> MSGSHHHHHHSSGIEGRGRLQTRQDVLYLYNWTYYTPTSLIKKFEQQYNVQVVYDDYASNEDMFAKLSIGASGYDLVVPSGDFVSIMKRKHLLEKIDLSKIPNVQFIKES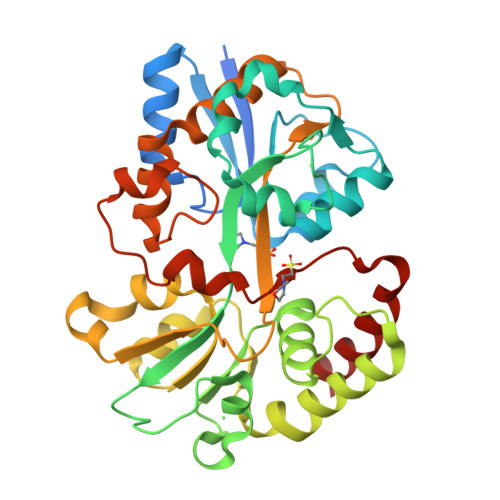VRARIAYDPKMEYSVPYYLGAAGIAVNKKAVPSYARTWSIFSRKDLAYRMSMMDDMREVMGAALASLGYNVNTKNEQELAQAAILVTDHWKPNLVKFDSDGYAKSFASGDFVVAHGFAEAFFAETPEAMHEHIDFFIPQDVASPVYVDSFCIPKGARNRDLAHAFINFFLEPAHYAEFLDTFGFPSTIHREAAAYQKKTPYYSEHDLERGTLKTDVGAAIEHYNAHWNAVRFR>MALEEIRPKEVYLDRKLLTLEDKELGSGNFGTVKKGYYQMKKVVKTVAVKILKNEANDPALKDELLAEANVMQQLDNPYIVRMIGICEAESWMLVMEMAELGPLNKYLQQNRHVKDKNIIELVHQVSMGMKYLEESNFVHRDLAARNVLLVTQHYAKISDFGLSKALRADENYYKAQTHGKWPVKWYAPECINYYKFSSKSDVWSFGVLMWEAFSYGQKPYR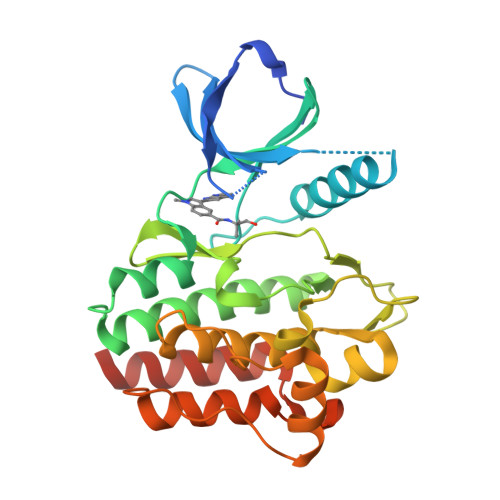GMKGSEVTAMLEKGERMGCPAGCPREMYDLMNLCWTYDVENRPGFAAVELRLRNYYYDVVNEGHHHHHH[2x]> SNAMAKTLKDLQGWEIITTDEQGNIIDGGQKRLRRRGAKTEHYLKRSSDGIKLGRGDSVVMHNEAAGTYSVYMIQELRLNTLNNVVELWALTYLRWFEVNPLAHYRQFNPDANILNRPLNYYNKLFSETANKNELYLTAELAELQLFNFIRVANVMDGSKWEVLKGNVDPERDFTVRYICEPTGEKFVDINIEDVKAYIKKVEPREAQEYLKDLTLPSKK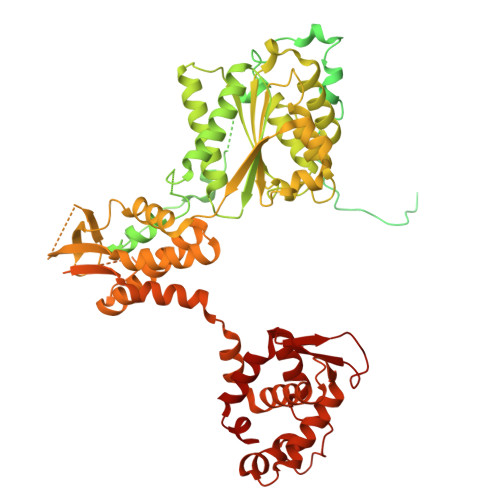KEIKRGPQKKDKATQTAQISDAETRATDITDNEDGNEDESSDYESPSDIDVSEDMDSGEISADELEEEEDEEEDEDEEEKEARHTNSPRKRGRKIKLGKDDIDASVQPPPKKRGRKPKDPSKPRQMLLISSCRANNTPVIRKFTKKNVARAKKKYTPFSKRFKSIAAIPDLTSLPEFYGNSSELMASRFENKLKTTQKHQIVETIFSKVKKQLNSSYVKEEILKSANFQDYLPARENEFASIYLSAYSAIESDSATTIYVAGTPGVGKTLTVREVVKELLSSSAQREIPDFLYVEINGLKMVKPTDCYETLWNKVSGERLTWAASMESLEFYFKRVPKNKKKTIVVLLDELDAMVTKSQDIMYNFFNWTTYENAKLIVIAVANTMDLPERQLGNKITSRIGFTRIMFTGYTHEELKNIIDLRLKGLNDSFFYVDTKTGNAILIDAAGNDTTVKQTLPEDVRKVRLRMSADAIEIASRKVASVSGDARRALKVCKRAAEIAEKHYMAKHGYGYDGKTVIEDENEEQIYDDEDKDLIESNKAKDDNDDDDDNDGVQTVHITHVMKALNETLNSHVITFMTRLSFTAKLFIYALLNLMKKNGSQEQELGDIVDEIKLLIEVNGSNKFVMEIAKTLFQQGSDNISEQLRIISWDFVLNQLLDAGILFKQTMKNDRICCVKLNISVEEAKRAMNEDETLRNL> KIKDPKILGIDPNVTQYTGYLDVEDEDKHFFFWTFESRNDPAKDPVILWLNGGPGCSSLTGLFFELGPSSIGPDLKPIGNPYSWNSNATVIFLDQPVNVGFSYSGSSGVSNTVAAGKDVYNFLELFFDQFPEYVNKGQDFHIAGESYAGHYIPVFASEILSHKDRNFNLTSVLIGNGLTDPLTQYNYYEPMACGEGGEPSVLPSEECSAMEDSLERCLGLIESCYDSQSVWSCVPATIYCNNAQLAPYQRTGRNVYDIRKDCEGGNLCYPTLQDIDDYLNQDYVKEAVGAEVDHYE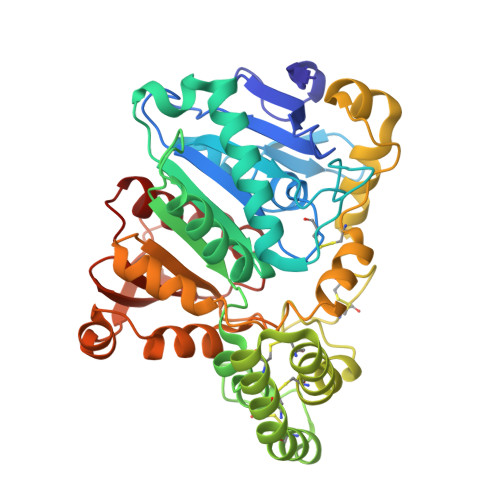SCNFDINRNFLFAGDWMKPYHTAVTDLLNQDLPILVYAGDKDFICNWLGNKAWTDVLPWKYDEEFASQKVRNWTASITDEVAGEVKSYKHFTYLRVFNGGHMVPFDVPENALSMVNEWIHGGFSL> VVRVADTMPSGPSNSESIPALTAAETGHTSQVVPS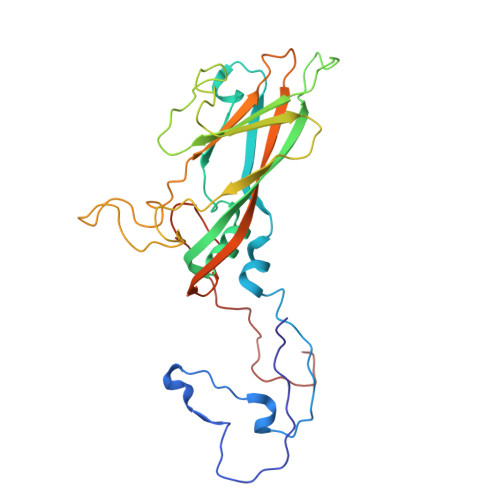DTIQTRHVRNFHVRSESSVENFLSRSACVYIVEYKTRDDTPDKMYDSWVINTRQVAQLRRKLEFFTYVRFDVEVTFVITSVQDDSTRQNTDTPALTHQIMYVPPGGPIPQAVDDYNWQTSTNPSVFWTEGNAPPRMSIPFMSVGNAYSNFYDGWSHFSQTGVYGFNTLNNMGKLYFRHVNDKTISPITSKVRIYFKPKHVKAWVPRPPRLCEYTHKDNVDFEPKGVTTSRTQLTISNSTH>[4x]MAEQVALSRTQVCGILREELFQGDAFHQSDTHIFIIMGASGDLAKKKIYPTIWWLFRDGLLPENTFIVGYARSRLTVADIRKQSEPFFKATPEEKLKLEDFFARNSYVAGQYDDAASYQRLNSHMNALHLGSQANRLFYLALPPTVYEAVTKNIHESCMSQIGWNRIIVEKPFGRDLQSSDRLSNHISSLFREDQIYRIDHYLGKEMVQNLMVLRFANRIFGPIWNRDNIACVILTFKEPFGTEGRGGYFDEFGIIRDVMQNHLLQMLCLVAMEKPASTNSDDVRDEKVKVLKCISEVQANNVVLGQYVGNPDGEGEATKGYLDDPTVPRGS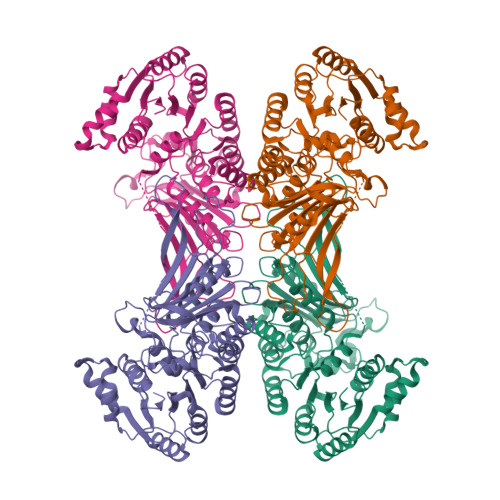TTATFAAVVLYVENERWDGVPFILRCGKALNERKAEVRLQFHDVAGDIFHQQCKRNELVIRVQPNEAVYTKMMTKKPGMFFNPEESELDLTYGNRYKNVKLPDAYERLILDVFCGSQMHFVRSDELREAWRIFTPLLHQIELEKPKPIPYIYGSRGPTEADELMKRVGFQYEGTYKWVNPHKLLEHHHHHH> MAKKTLPAGVKSPPYIFSPIPFLGHAIAFGKSPIEFLENAYEKYGPVFSFTMVGKTFTYLLGSDAAALLFNSKNEDLNAEDVYSRLTTPVFGKGVAYDVPNPVFLEQKKMLKSGLNIAHFKQHVSIIEKETKEYFESWGESGEKNVFE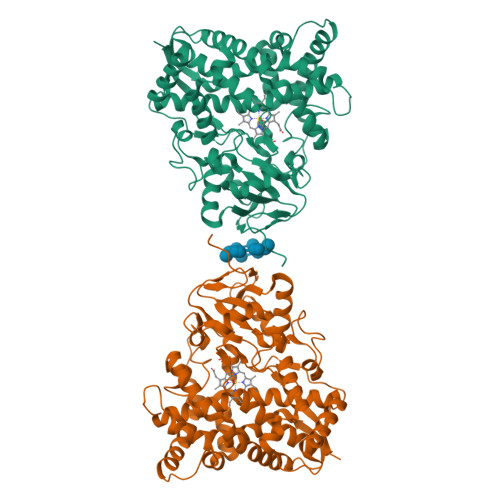ALSELIILTASHCLHGKEIRSQLNEKVAQLYADLDGGFSHAAWLLPGWLPLPSFRRRDRAHREIKDIFYKAIQKRRQSQEKIDDILQTLLDATYKDGRPLTDDEVAGMLIGLLLAGQHTSSTTSAWMGFFLARDKTLQKKCYLEQKTVCGENLPPLTYDQLKDLNLLDRCIKETLRLRPPIMIMMRMARTPQTVAGYTIPPGHQVCVSPTVNQRLKDSWVERLDFNPDRYLQDNPASGEKFAYVPFGAGRHRCIGENFAYVQIKTIWSTMLRLYEFDLIDGYFPTVNYTTMIHTPENPVIRYKRRSTHHHHHH>[2x]MPSNCRRFEGKVAIVTAATKGIGLAIAERLLDEGASVVIGSRNQKNVDEAIEYLKNKGLTKVAGIAGHIASTDDQKKLVDFTLQKFGKINILVNNHGINPAFGHILEVSDQVWDKLFEVNVKAGFQMTKLVHPHIAKEGGGAIIFNASYSAYKSPPGIAAYGVTK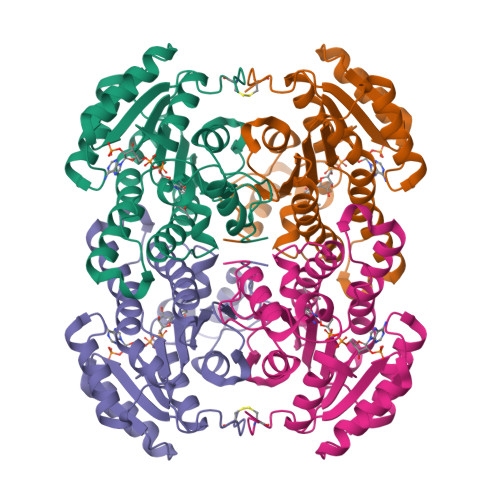TTLVGLTRALAMGLAKDNIRVNGIAPGVIKTKMSQVLWDGGEDAEKELTDIQEIALGRLGVPDDCAGTVAYLASDDSSYITGEMIIIAGGVQARL>[2x]MAAFSKYLTARNSSLAGAAFLLL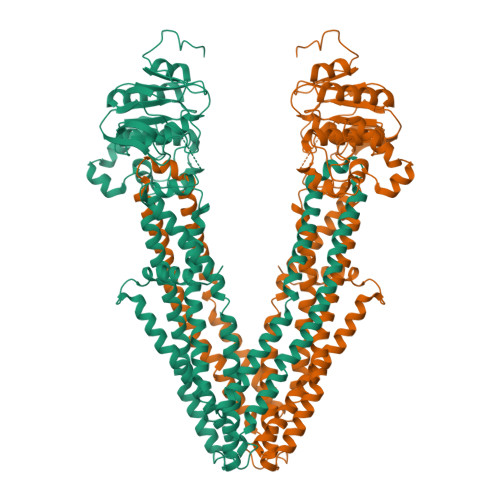CLLHKRRRALGLHGKKSGKPPLQNNEKEGKKERAVVDKVFFSRLIQILKIMVPRTFCKETGYLVLIAVMLVSRTYCDVWMIQNGTLIESGIIGRSRKDFKRYLLNFIAAMPLISLVNNFLKYGLNELKLCFRVRLTKYLYEEYLQAFTYYKMGNLDNRIANPDQLLTQDVEKFCNSVVDLYSNLSKPFLDIVLYIFKLTSAIGAQGPASMMAYLVVSGLFLTRLRRPIGKMTITEQKYEGEYRYVNSRLITNSEEIAFYNGNKREKQTVHSVFRKLVEHLHNFILFRFSMGFIDSIIAKYLATVVGYLVVSRPFLDLSHPRHLKSTHSELLEDYYQSGRMLLRMSQALGRIVLAGREMTRLAGFTARITELMQVLKDLNHGKYERTMVSQQEKGIEGVQVIPLIPGAGEIIIADNIIKFDHVPLATPNGDVLIRDLNFEVRSGANVLICGPNGCGKSSLFRVLGELWPLFGGRLTKPERGKLFYVPQRPYMTLGTLRDQVIYPDGREDQKRKGISDLVLKEYLDNVQLGHILEREGGWDSVQDWMDVLSGGEKQRMAMARLFYHKPQFAILDECTSAVSVDVEGYIYSHCRKVGITLFTVSHRKSLWKHHEYYLHMDGRGNYEFKQITEDTVEFGSGSGLVPRGSGGGGSGGGGSGGHHHHHHHH>GSHMDPNTVSSFQVDCFLWHVRKRVADQELGDAPFLDRLRRDQKSLRGRGSTLGLDIETATRAG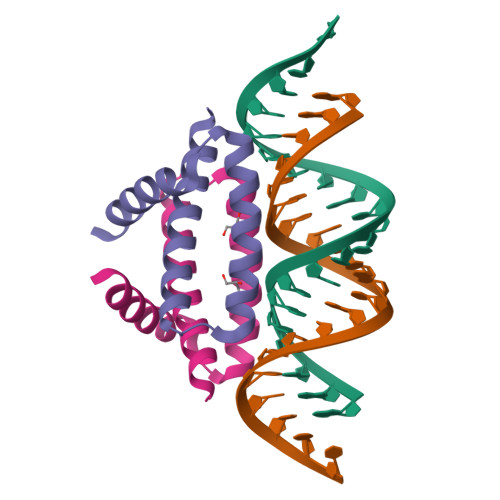KQIVERILK[2x]>CATGG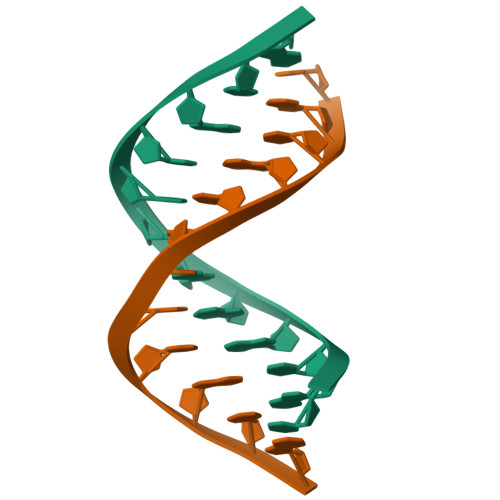GCCCATG[2x]> MAAVDIRDNLLGISWVDSSWIPILNSGSVLDYFSERSNPFYDRTCNNEVVKMQRLTLEHLNQMVGIEYILLHAQEPILFIIRKQQRQSPAQVIPLADYYIIAGVIYQAPDLGSVINSRVLTAVHGIQSAFDEAMSYCRYHPSKGYWWHFKDHEEQEKVKPKAKRKEEPSSIFQRQRVDALLIDLRQKFPPRFVQQKSGEKPVPVDQAKKEA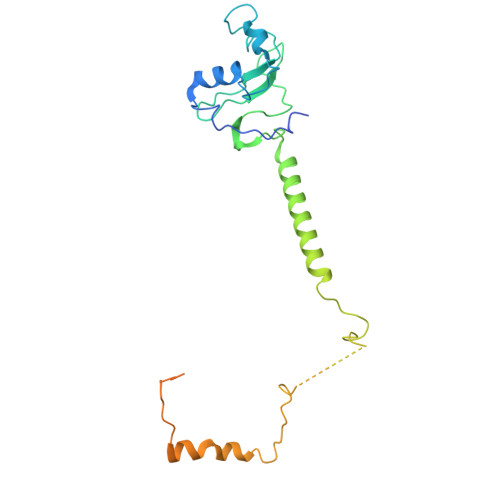EPLPETVKSEEKESTKNIQQTVSTKGPPEKRMRLQ>[6x]SNAQVSLNPEWLARNNDEHKIRRNDHRSPFQRDRARILHSAAFRRLQAKTQVHGT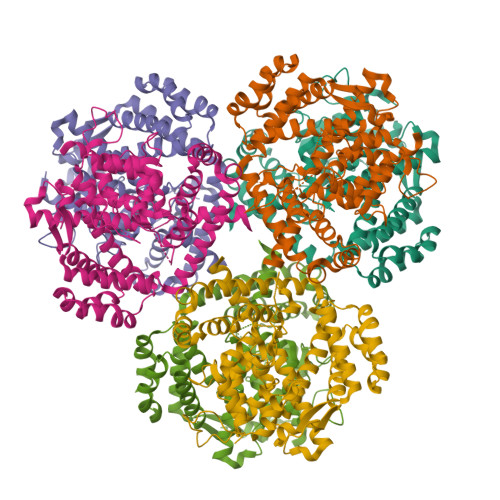SLNDFHRTRLTHSLEAAQIGTGIVAQIKLKQPEFRELLPSDSLIDSLCLAHDIGHPPYGHGGEIALNYMMRDHGGFEGNAQTFRIVTSLEPYTEHHGMNLSRRTLLGLLKYPALLSATRAAIPPPAVAHQRQLKAKDWSPAKGIYDCDLASLDWVLEPLCESDRELLGQMRAEPSSPKEHRKTRFKSLDCSIMELADDIAYGVHDLEDAIVLGMVTRAQWQEAAAAQLAECGDPWFEEHIAELSEMLFSGKHYVRKDAIGGIVNALLTSISVKPVEAPFHNELLAFNAYIEPHMGNALEVLKHFVSQYVIQIPQVQRFEYKGQQLIMDLFEALSADPERLLPQATGEKWRKAQEQDEGMRVICDYIAAMTDAYAQRLHQQLFSAQSHY> MVSQE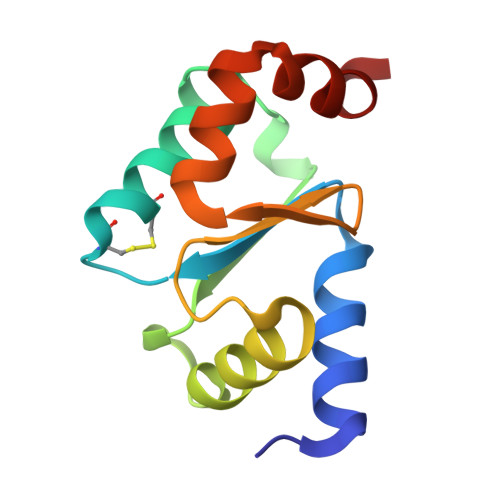TVAHVKDLIGQKEVFVAAKTYCPYCKATLSTLFQELNVPKSKALVLELDEMSNGSEIQDALEEISGQKTVPNVYINGKHIGGNSDLETLKKNGKLAEILKPVFQ>MRCIGISNRDFVEGVSGGSWVDIVLEHGSCVTTMAKNKPTLDFELIKTEAKQPATLRKYCIEAKLTNTTTESRCPTQGEPTLNEEQDKRFVCKHSMVDRGWGNGCGLFGKGGIVTCAMFTCKKNMEGKIVQPENLEYTVVITPHSGEEHAVGNDTGKHGKEVKITPQSSITEAELTGYGTVTMECSPRTGLDFNEMVLLQMKDKAWLVHRQWFLDLPLPWLPGADTQGSNWIQ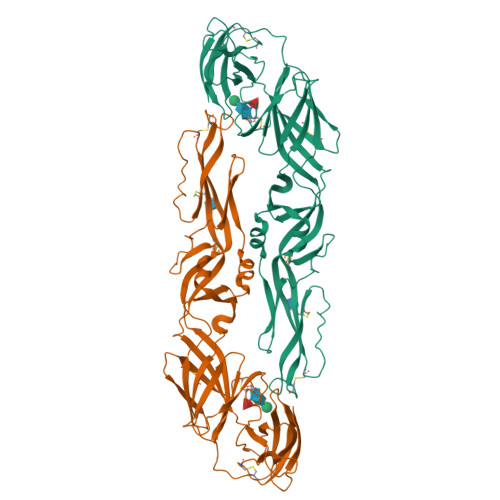KETLVTFKNPHAKKQDVVVLGSQEGAMHTALTGATEIQMSSGNLLFTGHLKCRLRMDKLQLKGMSYSMCTGKFKVVKEIAETQHGTIVIRVQYEGDGSPCKIPFEIMDLEKRHVLGRLITVNPIVTEKDSPVNIEAEPPFGDSYIIIGVEPGQLKLNWFKK[2x]Tegaserod | C16 H23 N5 O | 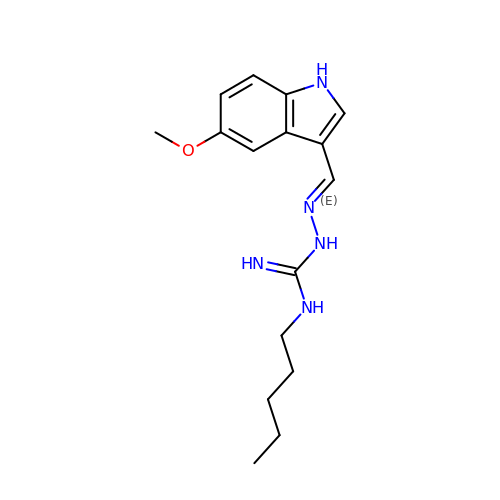IKBKZGMPCYNSLU-RGVLZGJSSA-N>MFNALVVDKDEESGKTQAAVKQLSLTDLPVGEVTVAVEYSTVNYKDGLCIGPGGGLVRKYPHVPGIDFAGTVENSSDERYK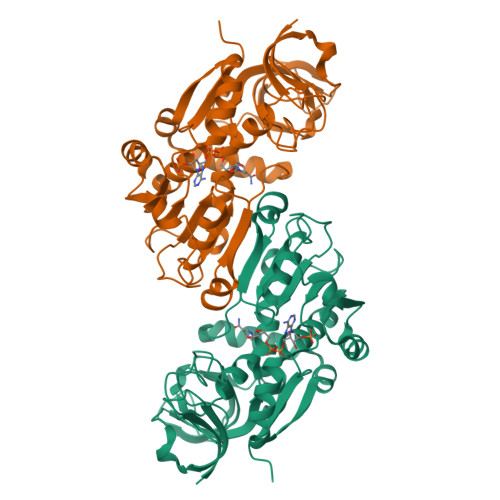PGDKVVLTGWRVGEAHWGGYSQKANVRADWLVPLPEGLDTRQAMAVGTAGFTAMLAVMALEDHGLTPGHGPVLVTGAAGGVGSVATAILAHLGYEVAAVTGRPETADYLTSLGATQIVARDEINETVKRPLESEIWAGCVDAVGGAMLARVLGQMKYGASVAAVGLAGGAGLPATVIPFLLRGVNLLGIDSVMQPYANRLRAWERIARDLPMDKLEAMIRPATLSDLPGLGADILKGQVQGRVVVDVNAH[2x]> MVTLEYNANSKLITASDAVVALSTETNIDQINVLT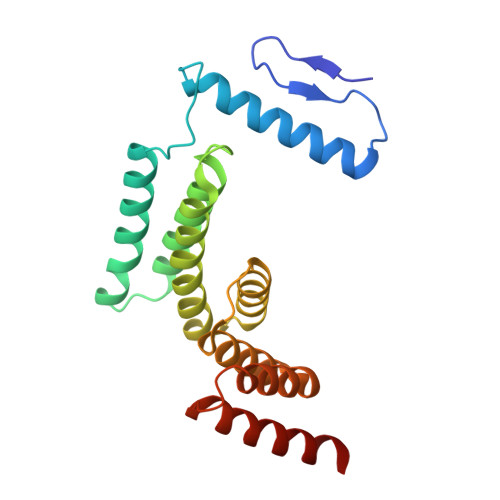TSLIGETNPNFTPQPNEALSKMIKGLFESGMKNLQQKKLNEALKNVSLAIEMAQRKRAPWEAFAIQLPELHFMLRSKIDLCLILGKHLEALQDLDFLLGTGLIQPDVFVRKADCLLKLRQWEEARATCERGLALAPEDMKLRALLIETARNLAEYNGE>MKKEETTTGPKETTIFAMHLGKALDPNLPVFVKAEKDTNIKLVNVASQNQTDQIQAYNLMLTEGKLPDIVSYELSADLENLGIEGGLIPLEDLINQHAPNLKKFFEENPRYKKDAVAVDGHIYMIPNYYDYFNIKVSQGYFIRQDWLEKLGLKEPRTVDELYTTLKAFREKDPNGNGKKDEVPFFVRANNVRKVLTSLVDLFKASPIWYEENGMVKYGPAQKEFKHAIKELSKWYKEGLIDEEIFTRGLESRDYLLSNNLGGATDDWIASTSSYNRN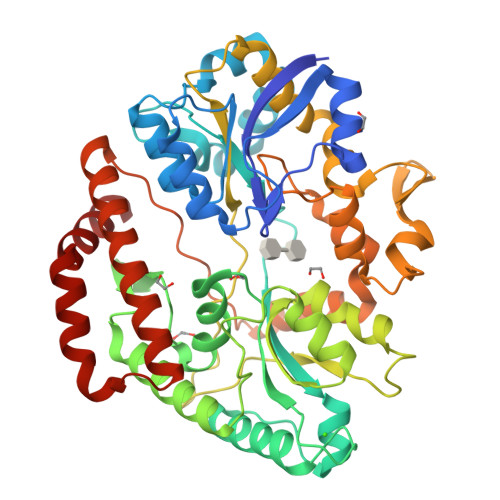LADKIPGFNLKLVLPYELNGNAKTRHARTTYLGGWGISKDAKDPVSLIKYFDYWYSVEGRRLWNFGIEGSEYTLVDGKPVFTDKVLKNPDGKTPLAVLREVGAQYRLGAFQDAQYELGWASESAKAGYKYYMDNDVVLDELPILKYTKEKSKEFVSIDTAMRAVVEEKAQQWILGSGDIDKEWDAYIKRLENLGLSKAEQIQNEAF[3x]>RVVCREASHAGSWYTASGPQLNAQLEGWLSQVQSTKRPARAIIAPHAGYTYCGSCAAHAYKQVDPSITRRIFILGPSHHVPLSRCALSSVDIYRTPLYDLRIDQKIYGELWKTGMFERMSLQTDEDEHSIEMHLPYTAKAMESHKDEFTIIPVLVGALSESKEQEFGKLFSKYLADPSNLFVVSSDFCHWGQRFRYSYYDESQGEIYRSIEHLDK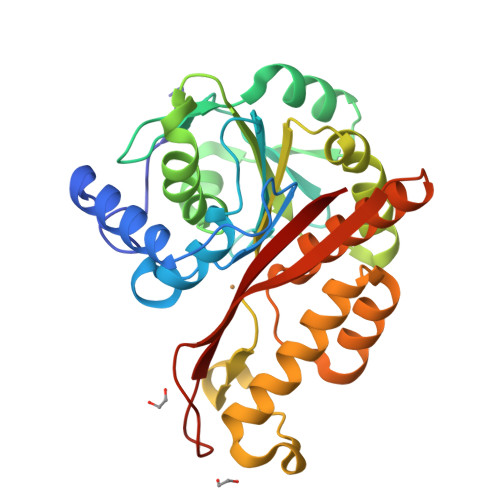MGMSIIEQLDPVSFSNYLKKYHNTICGRHPIGVLLNAITELQKNGMNMSFSFLNYAQSSQCRNWQDSSVSYAAGALTVH[4x]>MSDHGDVSLPPEDRVRALSQLGSAVEVNEDIPPRRYFRSGVEIIRMASIYSEEGNIEHAFILYNKYITLFIEKLPKHRDYKSAVIPEKKDTVKKLKEIAFPKAEELKAELLKRYTKEYTEYNEEKKKEAEELARNMAIQQELEKEK[2x];>[2x]KVTDALPEPE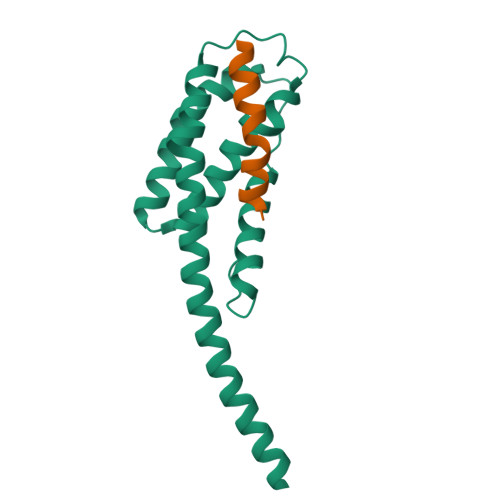PPGAMAASEDEEEEEEALEAMQSRLATLRS> AKWNPAGARRPVLDEAPVFYPTEEEFEDTLKYIESIRPMAEPYGICRIVPPSSWKPPCLLKDKSIWEGSKFSTRVQKVDKLQNRKSSKKGRRGGMMKRRKLAESEENSATAHTQTGMQQSPERFGFEPGPEFTLQTFQKYADDFSKQYFRKD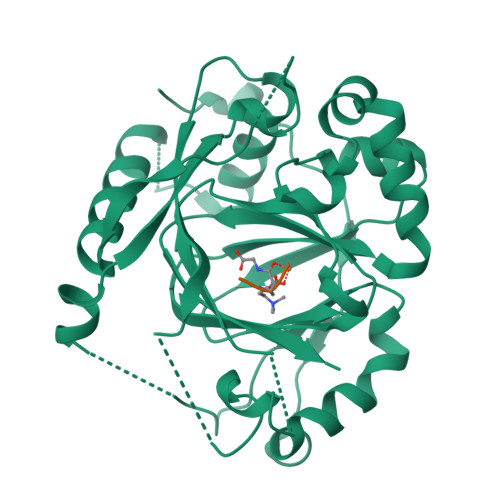TSMDSVPSVEDIEGEYWRIVEVPTEEIEVIYGADLETGTFGSGFPKLSPETKSDAEDKYAQSGWNLNNLPRLQGSVLSFEGGDISGVLVPWVYVGMCFSSFCWHVEDHHLYSLNYMHWGAPKLWYGVPGKDAVNLESAMRKHLPELFEEQPDLLHNLVTQFSPSLLKSEGVHVYRCVQHEGEFVLTFPRAYHAGFNCGFNCAEAVNVA;> TKQ> MAQLALALDTVTRYLRLKAPFAAFRPFQSGSFRSTTPVPSFSAVYGLLLNLAGIEQRQEVEGKVTLIKPKAELPKLAIAIGQVKPSSTSLINQQLHNYPVGNSGKEFASRTFGSKYWIAPVRREVLVNLDLIIGLQSPVEFWQKLDQGLKGETVINRYGLPFAGDNNFLFDEIYPIEKPDLASWYCPLEPDTRPNQGACRLTLWIDRENNTQTTIKVFSPSDFRLEPPAKAWQQLPG;>[7x]MSNLNLFATILTYPAPASNYRGESEENRSVIQKILKDGQKYAIISPESMRNALREMLIELGQPNNRTRLHSEDQLAVEFKEYPNPDKFADDFLFGYMVAQTNDAKEMKKLNRPAKRDSIFRCNMAVAVNPYKYDTVFYQSPLNAGDSAWKNSTSSALLHREVTHTAFQYPFALAGKDCAAKPEWVKALLQAIAELNGVAGGHARAYYEFAPRSVVARLTPKLVAGYQTYGFDAEGNWLELSRLTATDSDNLDLPANEFWLGGELVRKMDQEQKAQLEAMGAHLYANPEKLFAD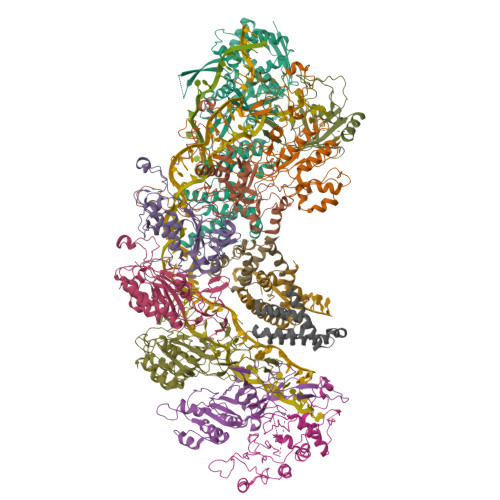LADSFLGV;> MPKTQAEILTLDFNLAELPSAQHRAGLAGLILMIRELKKWPWFKIRQKEKDVLLSIENLDQYGASIQLNLEGLIALFDLAYLSFTEERKSKSKIKDFKRVDEIEIEENGKNKIQKYYFYDVITPQGGFLAGWDKSDGQIWLRIWRDMFWSIIKGVPATRNPFNNRCGLNLNAGDSFSKDVESVWKSLQNAEKTTGQSGAFYLGAMAVNAENVSTDDLIKWQFLLHFWAFVAQVYCPYILDKDGKRNFNGYVIVIPDIANLEDFCDILPDVLSNRNSKAFGFRPQESVIDVPEQGALELLNLIKQRIAKKAGSGLLSDLIVGVEVIHAEKQGNSIKLHSVSYLQPNEESVDDYNAIKNSYYCPWFRRQLLLNLVNPKFDLASQSWLKRHPWYGFGDLLSRIPQRWLKENNSYFSHDARQLFTQKGDFDMTVATTKTREYAEIVYKIAQGFVLSKLSSKHDLQWSKCKGNPKLEREYNDKKEKVVNEAFLAIRSRTEKQAFIDYFVSTLYPHVRQDEFVDFAQKLFQDTDEIRSLTLLALSSQYPIKRQGETE;>MTVATTKTREYAEIVYKIAQGFVLSKLSSKHDLQWSKCKGNPKLEREYNDKKEKVVNEAFLAIRSRTEKQAFIDYFVSTLYPHVRQDEFVDFAQKLFQDTDEIRSLTLLALSSQYPIKRQGETE[3x]>[2x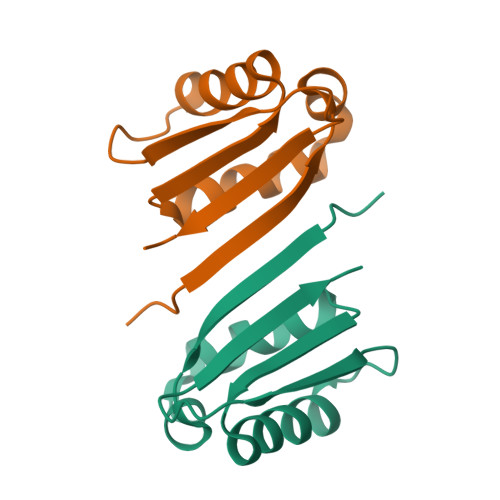]HHHHHHMDKLKDTPFMVQVKLPNYKDYLLDNKQVVLTFKLVHHSKKITLIGDANKILQYKNYFQANGARSDIDFYLQPTLNQKGVVMIASNYNDNPNSKEKPQTFDVLQGSQPMLGANT> VQTKALSKATLTDLPERWENMPNLEQKEIADNLTERQKLPWKTLNNEEIKAAWYISYGEWGPR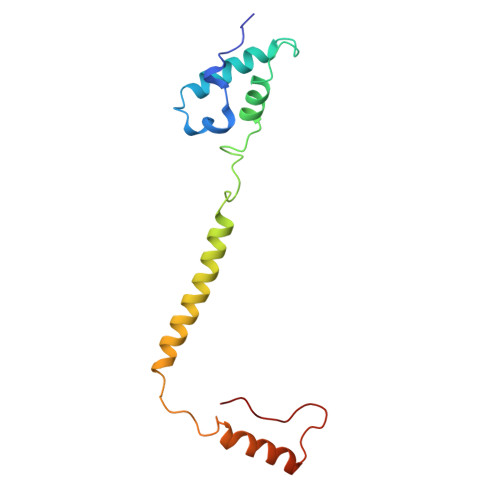RPVHGKGDVAFITKGVFLGLGISFGLFGLVRLLANPETPKTMNREWQLKSDEYLKSKNANPWGGYSQVQSK>SMHLTMPYVMPGDGEVVGVGEPVAIRFDENIADRGAAEKAIKITTNPPVEGAFYWLNNREVRWRPEHFWKPGTAVDVAVNTYGVDLGEGMFGEDNVQTHFTIGDEVIATADDNTKILTVRVNGEVVKSMPTSMGKDSTPTANGIYIVGSRYKHIIMDSSTYGVPVNSPNGYRTDVDWATQISYSGVFVHSAPWSVGAQGHT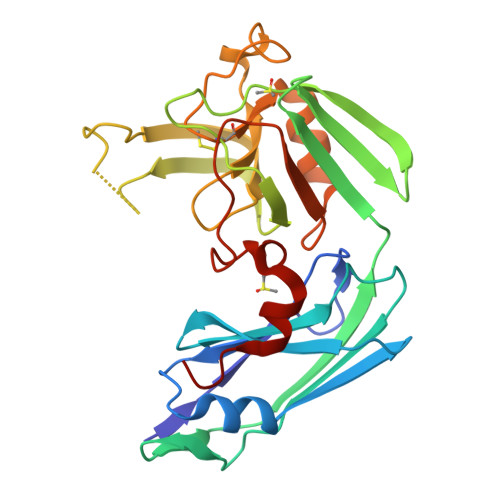NTSHGCLNVSPSNAQWFYDHVKRGDIVEVVNTVGGTLPGIDGLGDWNIPWDQWRAGNAKA[2x]> MKSNEHDDCQVTNPSTGHLFDLSSLSGRAGFTAAYSEKGLVYMSICGENENCPPGVGACFGQTRISVGKANKRLRYVDQVLQLVYKDGSPCPSKSGLSYKSVISFVCRPEAGPTNRPMLISLDKQTCTLFFSWHTPLACEQATECSVR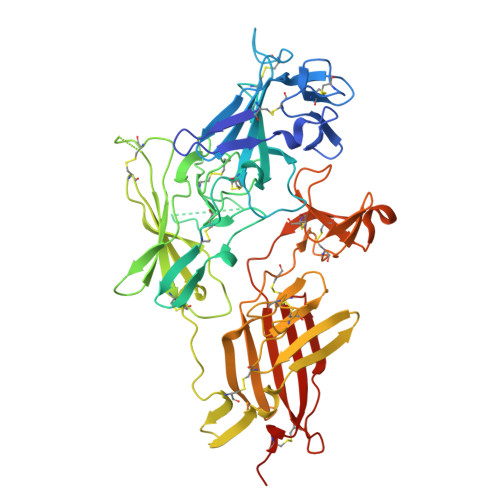NGSSIVDLSPLIHRTGGYEAYDESEDDASDTNPDFYINICQPLNPMHAVPCPAGAAVCKVPIDGPPIDIGRVAGPPILNPIANEIYLNFESSTPCLADKHFNYTSLIAFHCKRGVSMGTPKLLRTSECDFVFEWETPVVCPDEVRMDGCTLTDEQLLYSFNLSSLSTSTFKVTRDSRTYSVGVCTFAVGPEQGGCKDGGVCLLSGTKGASFGRLQSMKLDYRHQDEAVVLSYVNGDRCPPETDDGVPCVFPFIFNGKSYEECIIESRAKLWCSTTADYDRDHEWGFCRHSNSYRTSSIIFKCDEDEDIGRPQVFSEVRGCDVTFEWKTKVVCPPKKLKHHHHHH>[2x]DSTTQTTEQSKKNNDKPQDVITTSEIRKLNEKEPVYIYTSAAGGGFHMIPRTARLCTILTANRIPFTYRDLGTDDEARKVWKTFSKGRSLPGVVRGHNDLIGNWEEIEEANEDYKLRELIYDTI

Here we report a previously unknown budding yeast polarisome protein encoded by YFR016C, named actin-interacting protein 5 (Aip5). Aip5 is found to accelerate the formation of actin filaments in vitro through its C-terminal folded-domain (Aip5-C) and mediates actin cable assembly in cells. Structural studies by X-ray crystallography and biochemical assays have identified that Aip5-C is in a dimeric form, in which the dimer state and a loop region that directly binds to G-actin play essential roles in regulating actin assembly activity. Here we report a polarisome protein Aip5 that aids in actin assembly in vitro and promotes formin Bni1-mediated actin nucleation directly through the interactions toward G-actin and the C-terminus of Bni1.

L1150 in the loop region is highly conserved among multiple pathogenic filamentous fungi homologs. To test the L1150 role in actin filament assembly, we generated a protein mutant Aip5-C-L1150A and additional mutations of the amino acids adjacent to the loop region, single mutants Aip5-C-N1162A and Aip5-C-S1165C, and one triple mutant Aip5-C-3m (L1150A, N1162A, S1165C). Of the three single mutants, Aip5-C-L1150A showed the most drastic reduction in the polymerization rate. Notably, the additional S1165C and N1162A mutations to L1150A (Aip5-C-3m) resulted in complete suppression of the actin assembly activity of Aip5-C. To understand the consequences of the triple mutation, Aip5-C-3m was crystallized, and the structure was determined through molecular replacement using the native Aip5-C structure as the search model. Superposition of protomer A of Aip5-C and Aip5-C-3m structures showed an RMSD of 2.75 Å, which revealed missing electron density for the loop in Aip5-C-3m, indicating increased loop flexibility, whereas the superposition of protomer B showed an RMSD of 1.88 Å, which showed more similar conformations inside the well-folded region of Aip5-C. The Aip5-C-3m still formed a homodimer, however, and displayed significant conformational change when superposed with the native Aip5-C dimer. The hydrophobic contact established between two L1150 sites of Aip5-C promoters is, however, absent in the Aip-5-C-3m dimer. Furthermore, the loop sites in both protomers are far apart, with the heads of α1s pointing in opposite directions. Structural comparisons between Aip5-C and Aip5-C-3m suggest that the flexibility and/or the position of the loop plays a critical role in its actin assembly activities.> MSVDPNQYYKIRSQAIHQLKVNGEDPYPHKFHVDISLTDFIQKYSHLQPGDHLTDITLKVAGRIHAKRASGGKLIFYDLRGEGVKLQVMANSRNYKSEEEFIHINNKLRRGDIIGVQGNPGKTKKGELSIIPYEITLLSPCLHMLPHLHFGLKDKETRYRQRYLDLILNDFVRQKFIIRSKIITYIRSFLDELGFLEIETPMMNIIPGGAVAKPFITYHNELDMNLYMRIATELYHKMLVVGGIDRVYEIGRVFRNEGIDLTHNPEFTSCEFYMAYADYHDLMEIT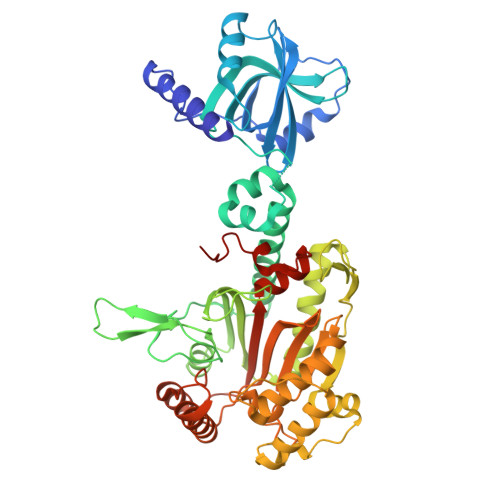EKMVSGMVKHITGSYKVTYHPDGPEGQAYDVDFTPPFRRINMVEELEKALGMKLPETNLFETEETRKILDDICVAKAVECPPPRTTARLLDKLVGEFLEVTCINPTFICDHPQIMSPLAKWHRSKEGLTERFELFVMKKEICNAYTELNDPMRQRQLFEEQAKAKAAGDDEAMFIDENFCTALEYGLPPTAGWGMGIDRVAMFLTDSNNIKEVLLFPAMKPEDKKEN4-[6-(3-hydroxyphenyl)pyrazin-2-yl]benzoic acid | C17 H12 N2 O3 | 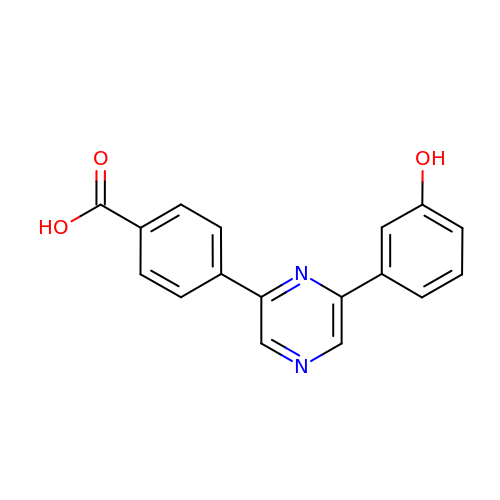RUXBJTDGOHITBG-UHFFFAOYSA-N>DESADIIYQFHSFEDIIQLSESLQRIGITGGTVYHYDGQYFLSLEDLGSHTAEGVVAVLAEYGNPTTLTIYRLQEYGKLIMD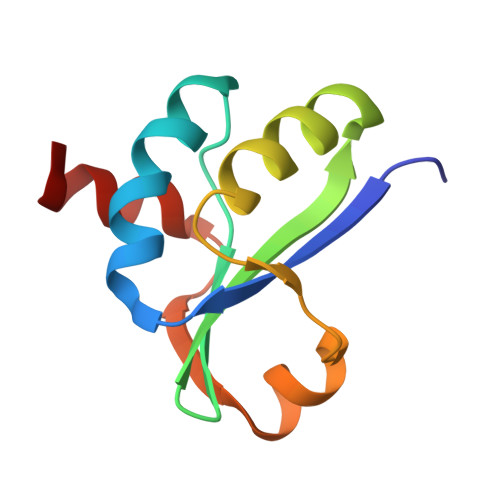GNAVETIQTHFS[6x]> MTLNKTDRIVITLG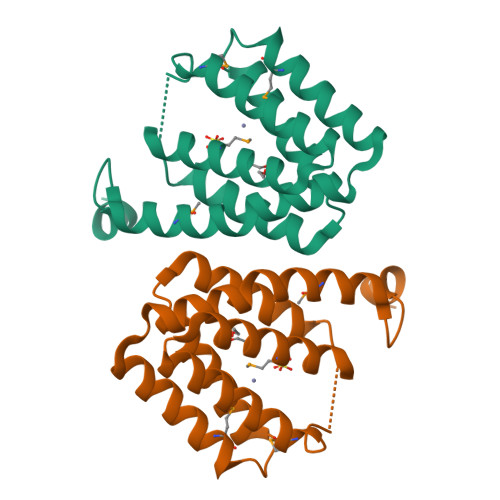KQIVHGKYVPGSPLPAEAELCEEFATSRNIIREVFRSLMAKRLIEMKRYRGAFVAPRNQWNYLDTDVLQWVLENDYDPRLISAMSEVRNLVEPAIARWAAERATSSDLAQIESALNEMIANNQDREAFNEADIRYHEAVLQSVHNPVLQQLSIAISSLQRAVFERTWMGDEANMPQTLQEHKALFDAIRHQDGDAAEQAALTMIASSTRRLKEIT> GQLAPGITMSEIDRIAQNIIKSHLETCQYTMEELHQLAWQTHTYEEIKAYQSKSREALWQQCAIQITHAIQYVVEF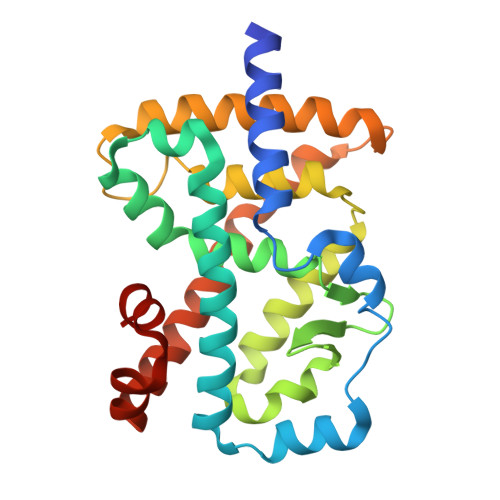AKRITGFMELCQNDQILLLKSGCLEVVLVRMCRAFNPLNNTVLFEGKYGGMQMFKALGSDDLVNEAFDFAKNLCSLQLTEEEIALFSSAVLISPDRAWLLEPRKVQKLQEKIYFALQHVIQKNHLDDETLAKLIAKIPTITAVCNLHGEKLQVFKQSHPDIVNTLFPPLYKELFNP2-(1,1-difluoroethyl)-5-methyl-N-[4-(pentafluoro-lambda~6~-sulfanyl)phenyl][1,2,4]triazolo[1,5-a]pyrimidin-7-amine 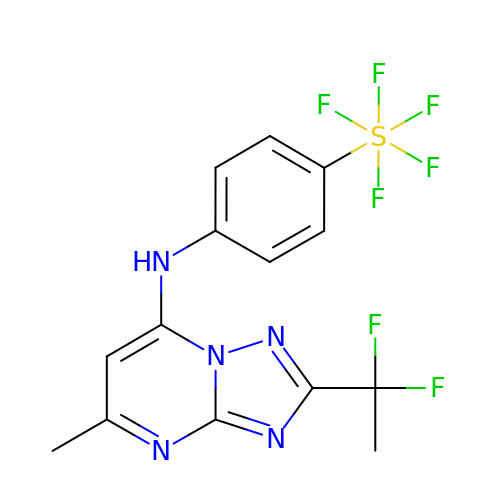| C14 H12 F7 N5 S | OIZSVTOIBNSVOS-UHFFFAOYSA-N> MGYTRERTNRHFFVSRANAFFSRLPISRIQRALAMEAIKKGSMKPWKHTKEQIIGSPITCNFEYNPRPVRLIGTVMDAHTEETSIKGGLKVYARSEEANMMLWIPAGNPKLKYEVTAAKGSFEHYLDERSKWDEAWLTGRA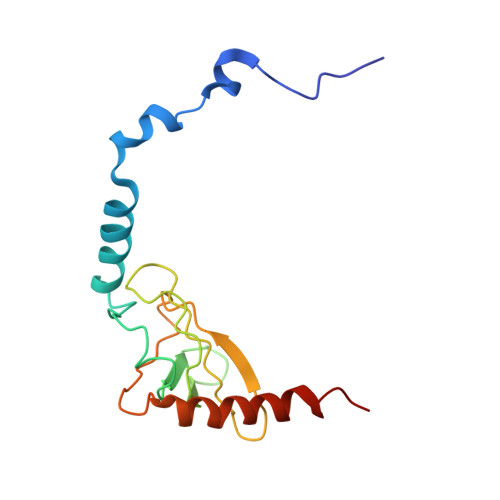RMK>SQAAAKVDVEFDYDGPLMKTEVPGPRSRELMKQLNIIQNAEAVHFFCNYEESRGNYLVDVDGNRMLDLYSQISSIPIGYSHPALVKLVQQPQNVSTFINRPALGILPPENFVEKLRESLLSVAPKGMSQLITMACGSCSNENAFKTIFMWYRSKERGQSAFSKEELETCMINQAPGCPDYSILSFMGAFHGRTMGCLATTHSKAIHKIDIPSFDWPIAPFPRLKYPLEEFVKENQQEEARCLEEVEDLIVKYRKKKKTVAGIIVEPIQSEGGDNHASDDFFRKLRDISRKHGCAFLVDEVQTGGGSTGKFWAHEHWGLDDPADVMTFSKKMMTGGFFHKEEFRPNAPYRI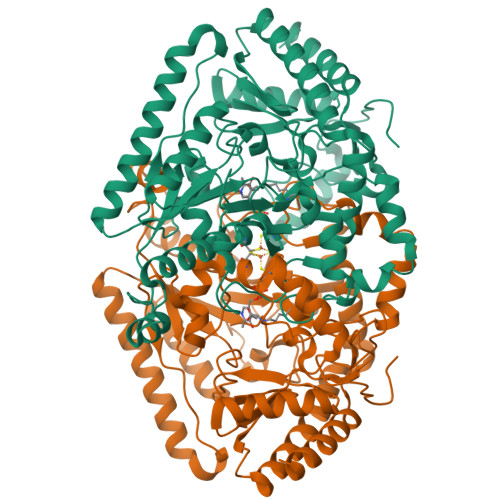FNTWLGDPSKNLLLAEVINIIKREDLLSNAAHAGKVLLTGLLDLQARYPQFISRVRGRGTFCSFDTPDESIRNKLISIARNKGVMLGGCGDKSIRFRPTLVFRDHHAHLFLNIFSDILADFK[4x]>EGVDISPKQDEGVLKVIKREGTGTEMPMIGDRVFVHYTGWLLDGTKFDSSLDRKDKFSFDLGKGEVIKAWDIAIATMKVGEVCHITCKPEYAYGSAGSPPKIPPNATLVFEVELFEFKGEDLTEEEDGG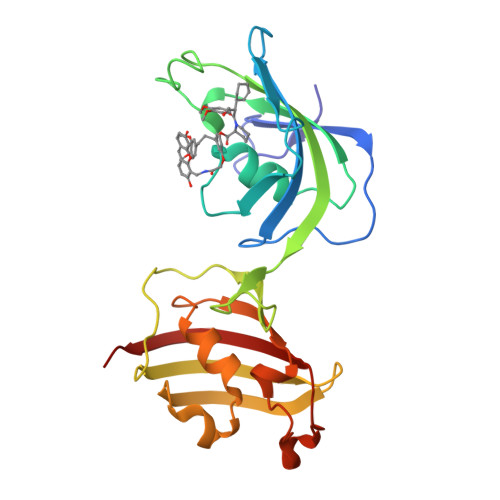IIRRIQTRGEGYAKPNEGAIVEVALEGYYKDKLFDQRELRFEIGEGENLDLPYGLERAIQRMEKGEHSIVYLKPSYAFGSVGKEKFQIPPNAELKYELHLKSFEKA[2x]>[2x]MRNQDKRAAHKDSEPSTEVNHTASSYQGRQQETGMNLRGIDGNEPTEGSNLLNNNEKMQGTPAEPNHLQRRRQIHACPPRGLLARVITNVTMVILLWAVVWSVTGSECLPGGNLFGIIMLFYCAIIGGKLFGLIKLPTLPPLPPLLGMLLAGFLIRNVPVISDNIQIKHKWSSALRSIALSVILVRAGLGLDSNALKKLKGVCVRLSLGPCLIEACTSAVLAYFLMGLPWQWGFMLGFVLGAVSPAVVVPSMLLLQEGGYGVEKGIPTLLMAAGSFDDILAITGFNTCLGMAFSTGSTVFNVLKGVLEVIIGVVTGLVLGFFIQYFPSSDQDNLVWKRAFLVLGLSVLAVFSSTYFGFPGSGGLCTLVTAFLAGRGWASTKTDVEKVIAVAWDIFQPLLFGLIGAEVLITALRPETIGLCVATLGIAVLIRILVTYLMVCFAGFNIKEKIFISFAWLPKATVQAAIGSVALDTARSHGEKQLEGYGMDVLTVAFLSIIITAPVGSLLIGLLGPRLLQKAEQNKDEEDQGETSIQV

The Na+/H+ exchanger SLC9B2, also known as NHA2, correlates with the long-sought-after Na+/Li+ exchanger linked to the pathogenesis of diabetes mellitus and essential hypertension in humans. Here we report the cryo-EM structures of bison NHA2 in detergent and in nanodiscs, at 3.0 and 3.5 Å resolution, respectively. NHA2 consists of 14 transmembrane (TM) segments, rather than the 13 TMs previously observed in mammalian Na+/H+ exchangers (NHEs) and related bacterial antiporters. The additional N-terminal helix in NHA2 forms a unique homodimer interface with a large intracellular gap between the protomers, which closes in the presence of phosphoinositol lipids.

The bison NHA2 construct used for structural studies is referred to as NHA2ΔN, because it does not include the first 69 residues of the N-terminal tail. The bison NHA2ΔN sample preparation was subsequently optimized for grid preparation, cryo-EM data acquisition and structural determination at pH 8.0. The final cryo-EM map of NHA2ΔN in detergent was estimated at 3.0 Å (Fourier shell correlation (FSC) = 0.143 criterion), although protomer A was consistently better aligned than protomer B, and was therefore resolved at a higher resolution. Overall, the structure of NHA2ΔN in detergent has a model resolution at 4.2 Å (FSC = 0.5), which is reflected in the fact that some side chains in the core domain and the connecting TM6–TM7 loop could not be modeled, probably due to flexibility. The observed additional N-terminal helix TM –1 is part of the dimer domain in NHA2ΔN and is domain-swapped, mediating homodimerization by interacting with TM8 and the TM8–TM9 loop in the neighboring protomer. As a result of the tilted angle of TM –1 and the length of the connecting loop to TM1, the NHA2ΔN protomers are held apart by ~ 25 Å on the intracellular side. In NHA2ΔN, the dimerization contacts are small, made up solely from interactions between TM −1 in one protomer and TM8 in the other. Although NHA2ΔN homodimerization appears very different to any Na+/H+ exchanger observed so far, the NHA2ΔN monomer has a high degree of structural conservation with the outward-facing monomer of NapA, but with the additional TM −1 helix. Dynamic elastic modeling of the nanodisc NHA2ΔN structure shows that TM −1 is indeed flexible and can spontaneously adopt the position seen in the detergent structure.> RTPEMPVLENRAAQGDITAPGGARRLTGDQTAALRDSLSDKPAKNIILLIGDGMGDSEITAARNYAEGAGGFFKGIDALPLTGQYTHYALNKKTGKPDYVTDSAASATAWSTGVKTYNGALGVDIHEKDHPTILEMAKAAGLATGNVSTAELQDAVPAALVAHVTSRKCYGPSATSEKCPGNALEKGGKGSITEQLLNARADVTLGGGAKTFAETATAGEWQGKTLREQAQARGYQLVSDAASLNSVTEANQQKPLLGLFADGNMPVRWLGPK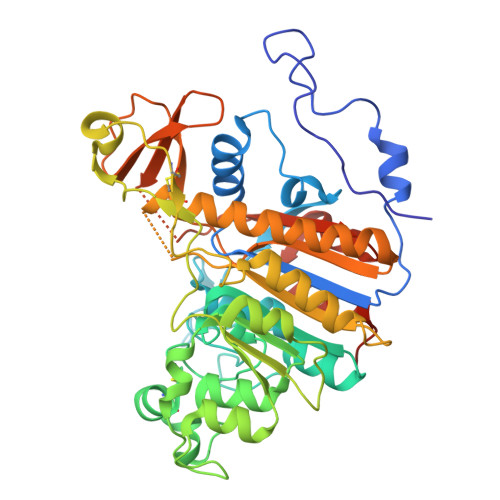ATYHGNIDKPAVTCTPNPQRNDSVPTLAQMTDKAIELLSKNEKGFFLQVEGASIDKQDHAANPCGQIGETVDLDEAVQRALEFAKKEGNTLVIVTADHAHASQIVAPDTKAPGLTQALNTKDGAVMVMSYGNSEEDSQEHTGSQLRIAAYGPHAANVVGLTDQTDLFYTMKAALGLKLEHHHHHH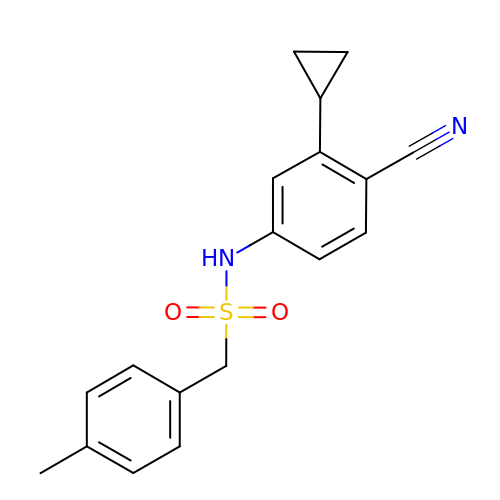N-(4-cyano-3-cyclopropylphenyl)-1-(4-methylphenyl)methanesulfonamide | C18 H18 N2 O2 S | PVSUTUAFYDGUTJ-UHFFFAOYSA-N> CFTPESTALLESGVRKPLGELSIGDRVLSM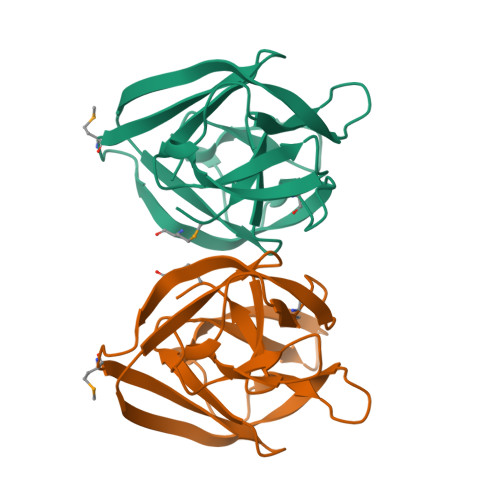TANGQAVYSEVILFMDRNLEQMQNFVQLHTDGGAVLTVTPAHLVSVWQPESQKLTFVFADRIEEKNQVLVRDVETGELRPQRVVKVGSVRSKGVVAPLTREGTIVVNSVAASCYA>AQDMVSPPPPIADEPLTVNTGIYLIESYSLDDCAETFKVNAFLSLSWKDRRLAFDPVRSGVRVKTYEPEAIWIPEIRFVNVENARDADVVDISVSPDGTVQYLERFSARVLSPLDFRRYPFDSQ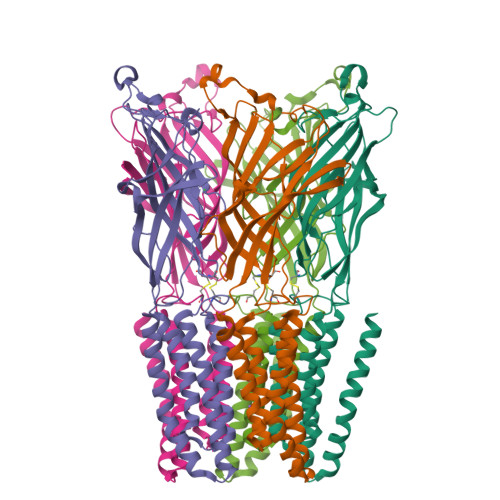TLHIYLIVRSVDTRNIVLAVDLEKVGKNDDVFLTGWDIESFTAVVKPANFALEDRLESKLDYQLRISRQYFSYIPNIILPMLFILFISWTAFWSTSYEANVTLVVSTLIAHIAFNILVETNCPKTPYMTYTGAIIFMIYLFYFVAVIEVTVQHYLKVESQPARAASITRASRIAFPVVFLLANIILAFLFFGF[5x]5'-deoxy-5'-({[2-(2,3-dihydroxyphenyl)ethyl]sulfonyl}amino)adenosine 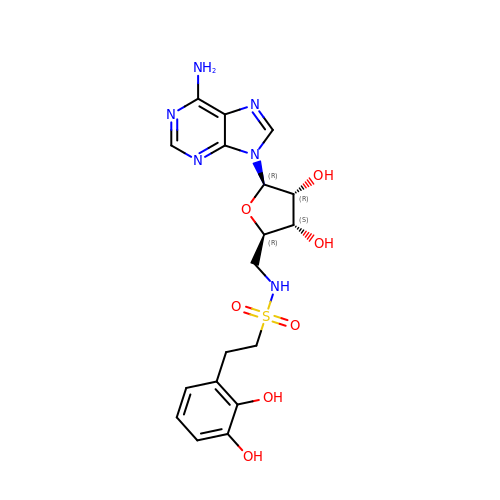| C18 H22 N6 O7 S | JESVQFVPCGDKBX-XKLVTHTNSA-N>MTKNSSLLAEFPTCPRDEKDRPRVFTAASGAWLTDESGFRWIDFDNARGSILLGHGDPVVAEAVARAATGADGTATGWSRRVDAVLERLHALCGGEVVGLFRSGTAAVRAAVLAVREATGRPLLLSAGYHGYDPMWYPSEAPLEPNADGVVDFFFDLGLLRELLRAPERVAAVVVSPDH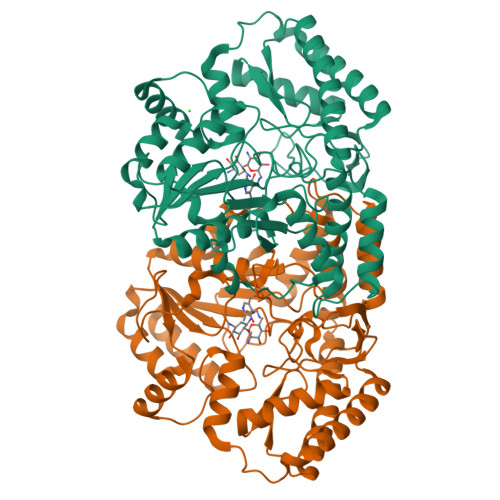MHLSPGWYRELRRLCSAAGVVLVADEVKVGLRYAPGLSTAELLAPDVWVVAKGMANGHAVSAVGGSRRLLKPLKEVSFTSFFEPTILAAADAALARVATGEPQRAVREAGDRFLRHARKALDDASLPVEIAGDGTFFQFVPATEELEEALYGAANAEGLLFYAGDNQGVSAAFDEAVLGEAERRFARVCERLAPYAGGEPVGDAARYRVAWNVMDGLRQAPRDREETTGLLARLLDDLEHHHHHH[8x]>[7x]MKIQMRNKKVLSFLTLTAIVSQALVYPVYAQTSTSNHSNKKKEIVNEDILPNNGLMGYYFTDEHFKDLKLMAPIKDGNLKFEEKKVDKLLDKDKSDVKSIRWTGRIIPSKDGEYTLSTDRDDVLMQVNTESTISNTLKVNMKKGKEYKVRIELQDKNLGSIDNLSSPNLYWELDGMKKIIPEENLFLRDYSNIEKDDPFIPNNNFFDPKLMSDWEDEDLDTDNDNIPDSYERNGYTIKDLIAVKWEDSFAEQGYKKYVSNYLESNTAGDPYTDYEKASGSFDKAIKTEARDPLVAAYPIVGVGMEKLIISTNEHASTDQGKTVSRATTNSKTESNTAGVSVNVGYQNGFTANVTTNYSHTTDNSTAVQDSNGESWNTGLSINKGESAYINANVRYYNTGTAPMYKVTPTTNLVLDGDTLSTIKAQENQIGNNLSPGDTYPKKGLSPLALNTM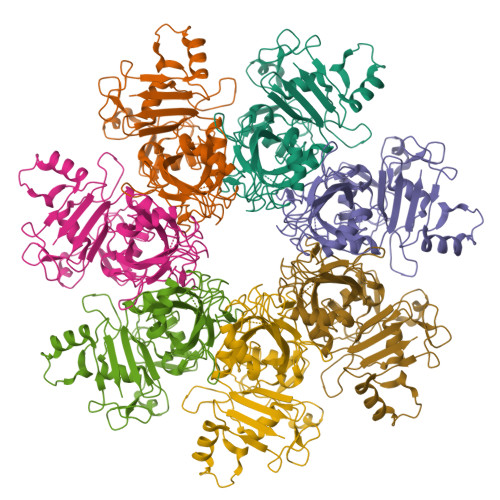DQFSSRLIAANYDQLKKLDAGKQIKLETTQVSGNFGTKNSSGQIVTEGNSWSDYISQIDSISASIILDTENESYERRVTAKNLQDPEDKTPELTIGEAIEKAFGATKKDGLLYFNDIPIDESCVELIFDDNTANKIKDSLKTLSDKKIYNVKLERGMNILIKTPTYFTNFDDYNNYPSTWSNVNTTNQDGLQGSANKLNGETKIKIPMSELKPYKRYVFSGYSKDPLTSNSIIVKIKAKEEKTDYLVPEQGYTKFSYEFETTEKDSSNIEITLIGSGTTYLDNLSITELNSTPEILDEPEVKIPTDQEIMDAHKIYFADLNFNPSTGNTYINGMYFAPTQTNKEALDYIQKYRVEATLQYSGFKDIGTKDKEMRNYLGDPNQPKTNYVNLRSYFTGGENIMTYKKLRIYAITPDDRELLVLSVD>[4x]SMAEIKQGIREVILCKDQDGKIGLRLKSIDNGIFVQLVQANSPASLVGLRFGDQVLQINGENCAGWSSDKAHKVLKQAFGEKITMTIRDRPFERTITMHKDSTGHVGFIFK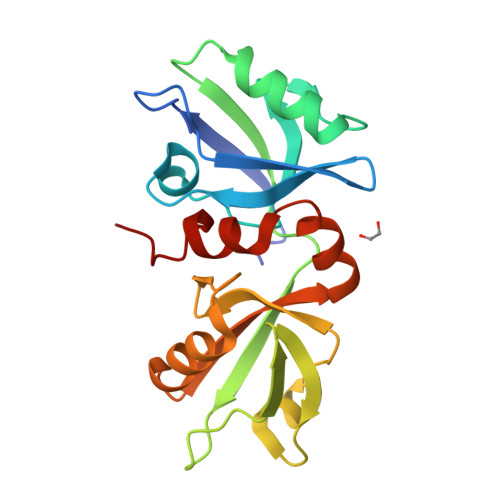NGKITSIVKDSSAARNGLLTEHNICEINGQNVIGLKDSQIADILSTSGTVVTITIMPAFIFEHIIKRMAPSIMKSLMDHTIPEV> MKTEWPELVGKSVAAAKK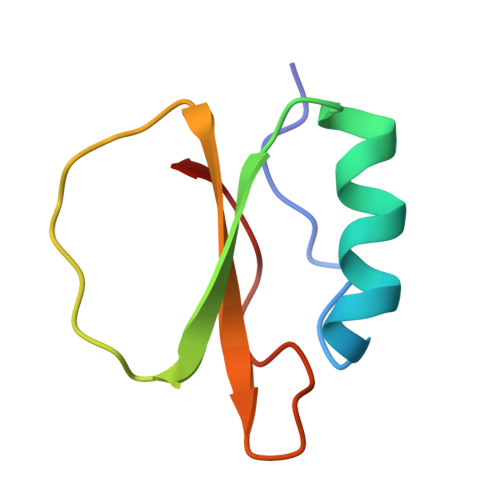VILQDKPEAQIIVLPVGTIVTMEYRIDRVRLFVDKLDNIAQVPRVG> MLRTHAAGSLRPADAGQTVTLAGWVARRRDHGGVIFIDLRDASGVSQVVFREGDVLAAAHRLRAEFCVAVTGVVEVRPEGNENPEIPTGQIEVNATELTVLGESAPLPFQLDEQAGEEARLKYRYLDLRREGPGNALRLRSKVNAAARSVLAEHDFVEIETPTLTRSTPEGARDFLVPARLQPGSFYALPQSPQLFKQLLMVAGMERYYQIARCYRDEDFRADRQPEFTQLDMEMSFVEADDVIAI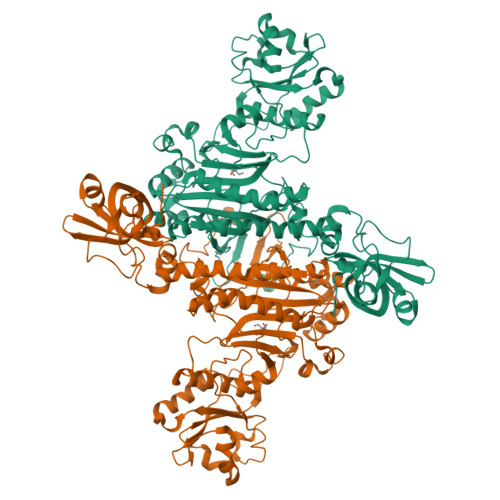SEQVLKAVWATIGYDLPLPLPRISYEEAMRRFGSDKPDLRFGIELVECTEYFKDTTFRVFQAPYVGAVVMPGGASQPRRTLDGWQEFAKQRGHKGLAYVLVGEDGTLGGPVAKNLSDAERDGLVAHVGANPGDCIFFAAGPAKGARALLGATRIEIAKRLDLIDPNAWAFTWVVDFPMFEAADEATAAGDVAVGSGAWTAMHHAFTAPKPDSVDTFDSDPGNALSDAYDIVCNGNEIGGGSIRIHRRDIQERVFAMMGIDHDEAQEKFGFLLDAFSYGAPPHGGIAFGWDRITALLAGVDSIREVIAFPKSGGGVDPLTDAPAPITPQQRKESGIDAKPREDKPKEDAKSKAAAALEHHHHHH>GAQRRNEIQVPDLDGYTTLKCDFHMHSVFSDGLVWPTVRVDEAYRDGLDAISLTEHIEYRPHKQDVVSDHNRSFDLCREQAEKLGILLIKGSEITRAMAPGHFNAIFLSDSNPLEQKDYKDAFREAKKQGAFMFWNHPGWDSQQPDTTKWWPEHTALYQEGCMHGIEVANGHLYMPEAIQWCLDKNLTMIGTSDIHQPIQTDYDFEKGEHRTMTFVFAKERSLQGIREALDNRRTAAYFHELLIGREDLLRPFFEKCVKIEEVSRNEQGVTLSITNVTDLVLKLKKTAHDTLLVYFRDMT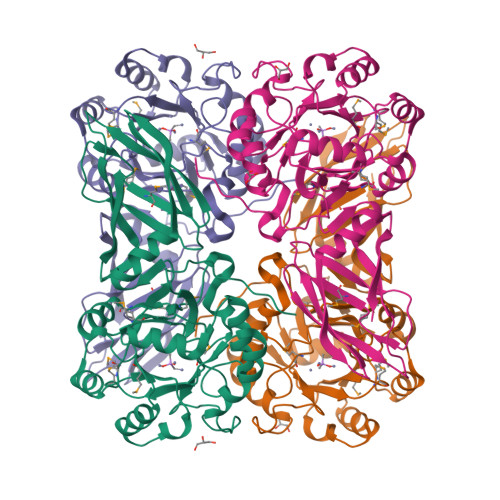LKPHTRYTVRIGFKQGIKGGDVNFEVTNFIVAPDKGLKYTISL[2x]>ESGAPPTDLQKMVMGNTKPVELILDGKTVAICCATGVFGTAYLVPRHLFAEQYDKIMLDGRAMTDSDYRVFEFEIKVKGQDMLSDAALMVLHRGNKVRDITKHFRDTARMKKGTPVVGVVNNADVGRLIFSGEALTYKDIVVSMDGDTMPGLFAYKAATRAGYAGGAVLAKDGADTFIVGTHSAGG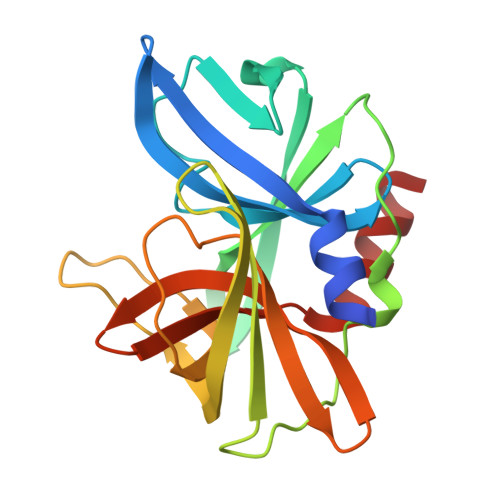NGVGYCSCVSRSMLQKMKAHVEH[2x]>MLKQVEIFTDGSALGNPGPG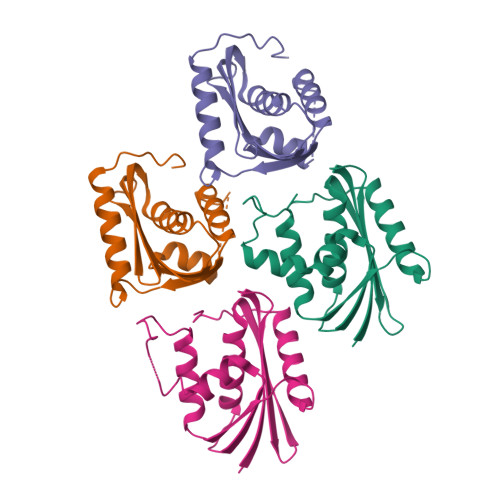GYGAILRYRGREKTFSAGYTRTTNNRMELKAAIEGLKALKEPAEVDLYTDSHYLKKAFTEGWLEGWRKRGWRTAEGKPVKNRDLWEALLLAMAPHRVRFHFVKGHAGHPENERADELARAAAMNPTLEDTGYQVEV[4x]2-[5-[5-ethanoyl-1-[(2~{R})-2-oxidanyl-3-[4-(2-oxidanylpropan-2-yl)piperidin-1-yl]propyl]-6,7-dihydro-4~{H}-pyrazolo[4,3-c]pyridin-3-yl]-2-(trifluoromethyl)phenyl]sulfanyl-1-pyrrolidin-1-yl-ethanone 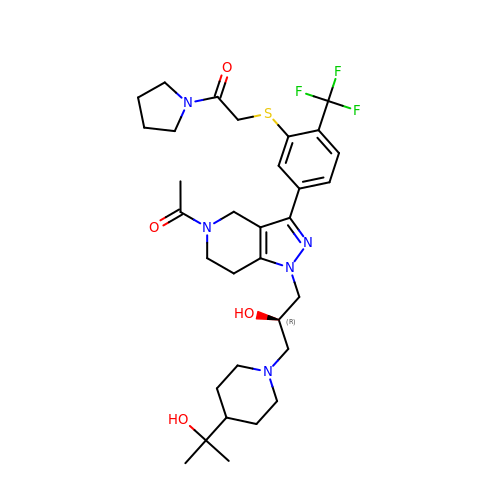| C32 H44 F3 N5 O4 S | QMRXULKWYQUBRF-XMMPIXPASA-N>MGHHHHHHSHKVQGAGQ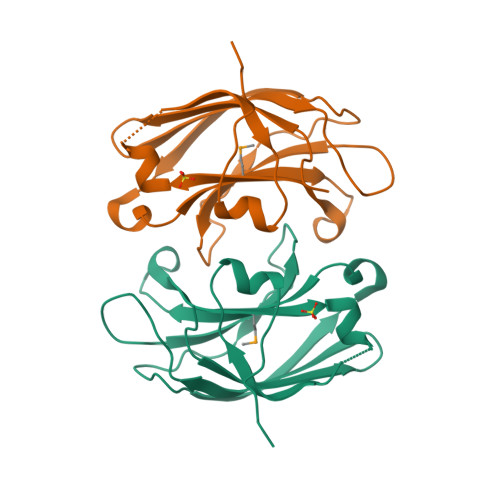LRLSIDAQDRVLLLHIIEGKGLISKQPGTCDPYVKISLIPEDSRLRHQKTQTVPDCRDPAFHEHFFFPVQEEDDQKRLLVTVWNRASQSRQSGLIGCMSFGVKSLLTPDKEISGWYYLLGEHLGRTKHLKVARRRL[2x]> GSIFSYRDGMRQSSLKKDWFLSEEEFKLWNRLYRLRDSDEIKEITLPQVQFSSLQNEENKPAQESTTGIHQLSLSEWRLWQD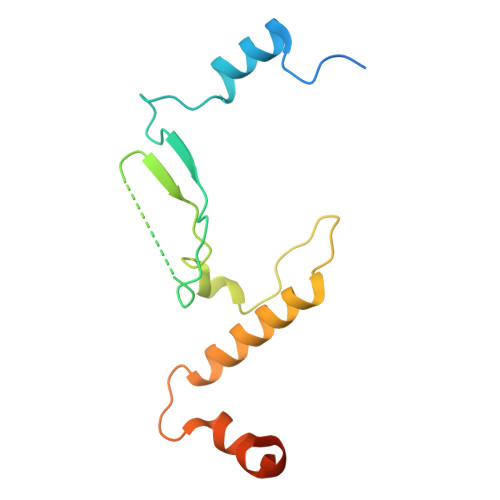HPLPTHQVDHSDRCRHFIGLMQMIEGMRHEEGECSYELEVESYLQMEDVTSTFIAPRNE> HHHHHHPGGSGAAVAPAAGQGSHSRQKKTFFLGDGQKLKDWHDKEAIRRDAQRVGNGEQGRPYPMTDAERVDQAYRENGFNIYVSDKISLNRSLPDIRHPNCNSKRYLETLPNTSIIIPFHNEGWSSLLRTVHSVLNRSPPELV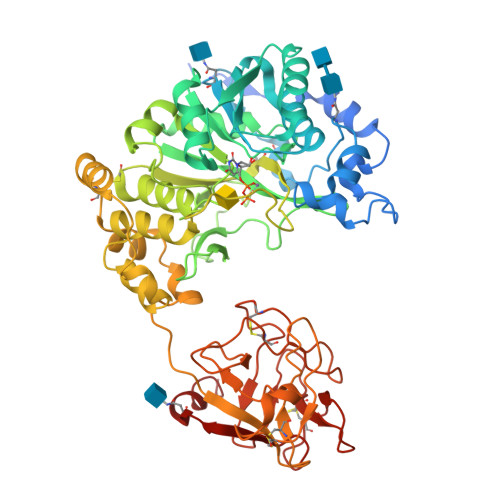AEIVLVDDFSDREHLKKPLEDYMALFPSVRILRTKKREGLIRTRMLGASVATGDVITFLDSHCEANVNWLPPLLDRIARNRKTIVCPMIDVIDHDDFRYETQAGDAMRGAFDWEMYYKRIPIPPELQKADPSDPFESPVMAGGLFAVDRKWFWELGGYDPGLEIWGGEQYEISFKVWMCGGRMEDIPCSRVGHIYRKYVPYKVPAGVSLARNLKRVAEVWMDEYAEYIYQRRPEYRHLSAGDVAVQKKLRSSLNCKSFKWFMTKIAWDLPKFYPPVEPPAAAWGEIRNVGTGLCADTKHGALGSPLRLEGCVRGRGEAAWNNMQVFTFTWREDIRPGDPQHTKKFCFDAISHTSPVTLYDCHSMKGNQLWKYRKDKTLYHPVSGSCMDCSESDHRIFMNTCNPSSLTQQWLFEHTNSTVLEKFNRN> SPCDTNWRY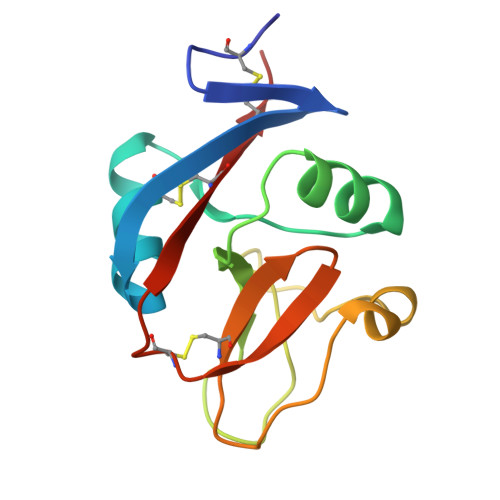YGDSCYGFFRHNLTWEESKQYCTDMNATLLKIDNRNIVEYIKARTHLIRWVGLSRQKSNEVWKWEDGSVISENMFEFLEDGKGNMNCAYFHNGKMHPTFCENKHYLMCERKAG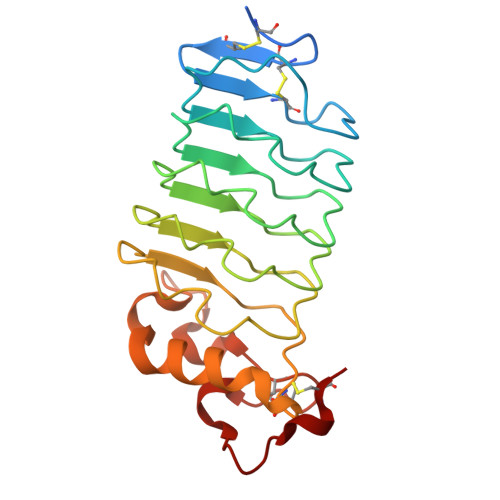> GGHHHHHHGSENLYFQGACPSQCSCSGTTVDCSGKSLASVPTGIPTTTQVLGLSSNQITKLEPGVFDSLVNLQILVLYQNQLTTLPAGVFDRLINLKELYFSNNQLTSLPAGVFDKLTQLTRLELQTNQLKSIPRGAFDNLKSLTNIYLFNNPWDCECSDILYLKNWIVQHASIVNPDGHGGVDNVKCSGTNTPVRAVTEASTSPSKCP> MAKGKSEVVEQNHTLILGWSDKLGSLLNQLAIANESLGGGTIAVMAERDKEDMELDIGKMEFDFKGTSVICRSGSPLILADLKKVSVSKARTIIVLAEDGNADQSDARALRTVLSLTGVKEGLRGHIVVEMSDLDNEVLVKLVGGDLVETVVAHDVIGRLMIQCARQPGLAQIWEDILGFENCEFYIKRWPQLDGMLFEDVLISFPAAIPCGIKVASYGGKIILNPDDSYVLQEGDEVLVIAEDDDTYAPAPLPMVRRGSLPKDFVYPKSPERILFCGWRRDMEDMITVLDASLAPDSELWMFNDVPEKEREKKLIDGGLDISRLENISLVNREGNAVIRRHLESLPLESFDSILILADESVEDSAIQADSRSLATLLLIRDIQARRLPYVAMASQTQGGNFSKGSWIGEMKQASDKTVIISEILDPRTKNLLSMSKISDYVLSNELVSMALAMVAEDRQINDVLEELFAEEGNEMHIRQADIYLREGEEMSFYEIMLRARQRREILIGYRLANAERAVINPPAKTGRRKWSLKDVFVVITEKEGSRSHHHHHH

Two DMI1 homologs, named POLLUX and CASTOR, were identified in L. japonicus and both of them are required to initiate symbiosis. To address these fundamental issues that define the primary function of these channels and their role in the symbiotic process, we performed functional characterization of the LjCASTOR channel and demonstrate that it functions as a Ca2+-regulated Ca2+ channel rather than as a K+ channel as previously proposed. We also determined the high-resolution crystal structure of the ligand-binding soluble domain of LjCASTOR and reveal that the entire soluble domain consists of two tandem RCK domains that assemble into a tetrameric gating ring where Ca2+ can bind and regulate the channel. Our high-resolution structure reveals multiple Ca2+-binding sites in the RCK gating ring and provides structural insights into Ca2+-regulated gating of CASTOR.

The CASTOR soluble domain was crystallized in the presence of Na+, Ca2+, and Mg2+, and its high-resolution structure allowed us to identify multiple bound ions clustered in two locations within each subunit. The protein crystals had a space group of I4 and contained one subunit per asymmetric unit; four crystallographic symmetry-related subunits assembled into a tetramer with the molecular fourfold coinciding with the crystallographic tetrad. The final structure was refined to 1.6 Å with an Rwork of 16.59% and an Rfree of 18.82%. Cluster I contains two bound ions and is located in the cleft between the two N-lobes. The other ion is defined as Ca2+ and is labeled as the Ca(I) site; it is coordinated by eight oxygen atoms including multiple negatively charged carboxylates, and it has ion–ligand distances of 2.4–2.5 Å, both of which are commonly seen for Ca2+ binding in proteins. The Ca2+ binding at the Ca(I) site mediates extensive interactions between the two N-lobes that lock them in a fixed position relative to each other. Cluster II sites are located in the cleft between the N- and C-terminal subdomains of RCK1 and contain three bound ions. The anomalous signals indicate that only two of the bound ions are Ca2+, labeled as Ca(II) and Ca(III) sites, respectively. The location of the two Ca2+ sites indicates that Ca2+ binding provides two tethering points between the N-lobe of RCK1 and the periphery C-terminal subdomains. The third ion in cluster II is in close proximity to the Ca(II) site and was identified as Na+ for two reasons: first, the bound ion has no anomalous diffraction signal; second, the bound ion has a coordination number of five with ion–ligand distances of 2.3–2.4 Å, which match that of the Na+ ion.5-mercaptopyridine-2,3-dicarboxylic acid | C7 H5 N O4 S | 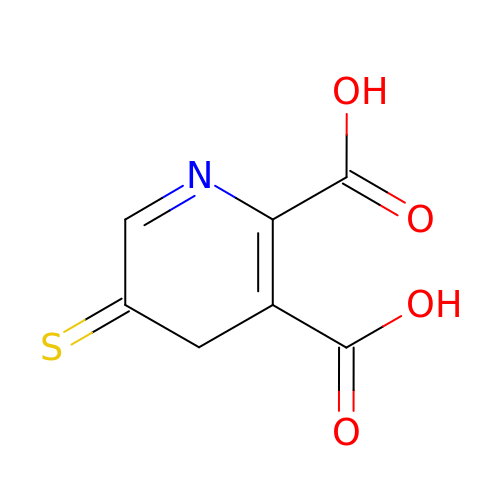XCYZNZIVHOIFRT-UHFFFAOYSA-N(6aS,7S,10aS)-8-hydroxy-4-methoxy-2,7,10a-trimethyl-5,6,6a,7,10,10a-hexahydrobenzo[h]quinazoline-9-carbonitrile | C17 H21 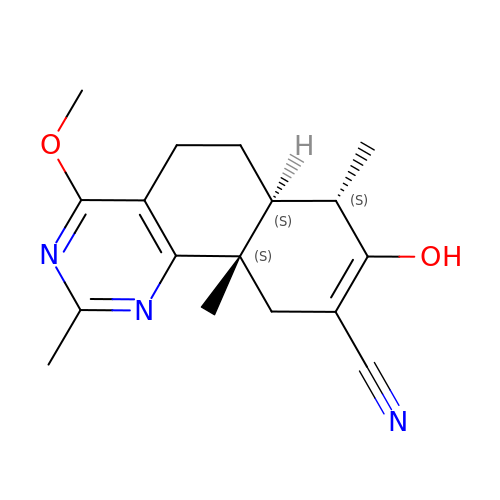N3 O2 | LBBXSDQROZEAQX-YHYSRRTLSA-N> GAMIESSTTIQVISAGLPRTGTKSLKNALEIIYHKPCYHMYEIIFNKQSDIIKWQNLIHDSHMITTPPPLTTKTIAIYDKLKELLDGYIATTDLPTCGFYKDLMNIYPNAKVLLTIRDKYDWLHSLRKVVLPKSNDPWKLKIEEGDKVLGLNSDFYKLTEDSLKFAFQKDDLNFDDDQVLLECYDEYNRLVQETVPSDRLLVLRLGDGWEPLCKFLNVEIPNGIDYPCVN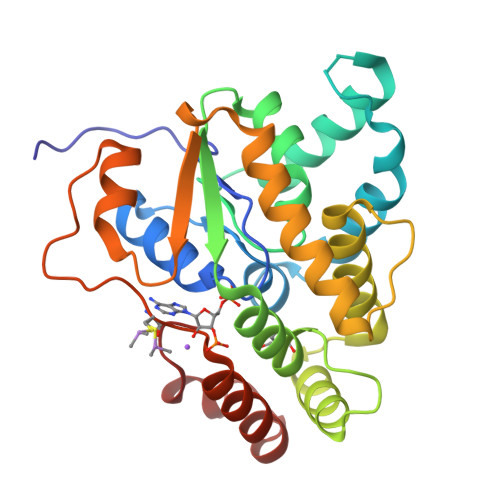SHHQMTQLTEQLIKYKSLDAIIHMFPDLI> MESRREEEITPVDILLQLVQMGKVDPWNIDIVDLTEKYIERLREMKELDLRVSARAILAASILVRMKSEA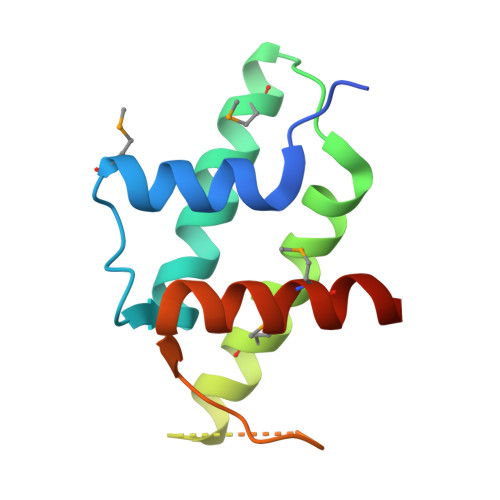LLYADEEDEEEKHEEHIRVEVEPLAPPLRRVERYYTFDDLLDALMDALEEAEKRKP2-amino-3-[(R)-{[(3S,4R,5R)-5-(2-amino-6-oxo-1,6-dihydro-9H-purin-9-yl)-4-hydroxyoxolan-3-yl]oxy}(hydroxy)phosphoryl]-1-[(S)-{[(3S,4R,5R)-5-(2-amino-6-oxo-1,6-dihydro-9H-purin-9-yl)-4-hydroxyoxolan-3-yl]oxy}(hydroxy)phosphoryl]-1H-imidazol-3-ium 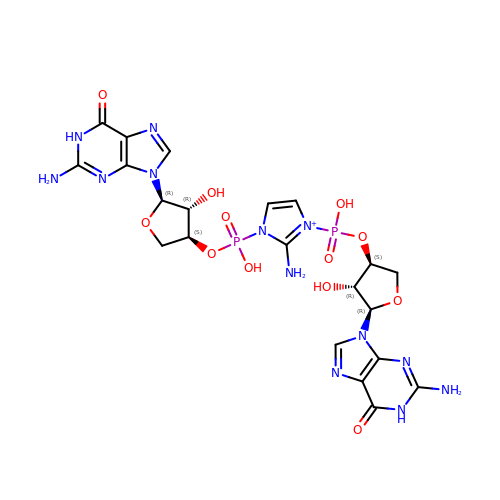| C21 H26 N13 O12 P2 | ZVPUVGSJWNSRDP-QIHYXNHISA-O Na+–K+–Cl− cotransporters functions as an anion importers, regulating trans-epithelial chloride secretion, cell volume, and renal salt reabsorption. Loop diuretics, including furosemide, bumetanide, and torsemide, antagonize both NKCC1 and NKCC2, and are first-line medicines for the treatment of edema and hypertension. Here we determined three cryo-EM structures of phosphorylated NKCC1 individually bound with furosemide, torsemide, and bumetanide, unlocking two modes of interaction of loop diuretics with NKCC1. In all the three co-structures, NKCC1 assembled as a C2-symmetric dimer in which two TMDs are separated by ~30 Å within the lipid bilayer and two cytosolic C-terminal domains (CTDs) interdigitate and associate extensively with the TMDs from beneath.

Furosemide intercalates into the NKCC1 extracellular ion entryway and assumes an extended configuration, with its sulfamoyl group facing the extracellular side and its furfuryl amine group reaching almost the midway of membrane. Notably, furosemide’s sulfamoylbenzoic moiety, which represents the molecular scaffold of carboxyl group-bearing loop diuretics, interacts extensively with residues in TM1, TM3, TM6, and TM8. Here, the chlorine atom barely contacts NKCC1, while the carboxyl group forms hydrogen bonds with Val302 and Met303 located on TM1b, and Ala497 residing on TM6a. The carboxyl group expels the Cl− ion from the so-called the Cl− site 1 and establishes ionic interaction with the K+ ion that was clearly seen to be co-occluded in the structure (Fig. EV3A). Further toward the midway of ion translocation path, furosemide’s furfuryl amine group is buried within a hydrophobic cavity and interacts with Met382 protruding from TM3, and IIe678, Ser679, and Phe682 which are all located on TM8. Indeed, we found that furosemide exhibits threefold higher potency in a K+ buffer than in a K+-free buffer. To settle this debate, we prepared pNKCC1 sample supplemented with 100 μM ATP and 2 mM furosemide, yielding an NKCC1/furosemide map in which we clearly observed a non-protein density that matches the shape of an ATP molecule in this cavity of NKCC1. In our pNKCC1/furosemide structure, ATP-Mg2+ binding stabilizes a loop (Gly925-Leu931) and a helix (Asn1002-Lys1021) that would otherwise be mobile and missing in all reported NKCC1 structures; the region which encompasses amino acids 932–1001 and contains sorting signals for trafficking NKCC1 to the basolateral membrane in epithelia remains unresolved. Our pNKCC1/furosemide map unambiguously defined the elusive N-terminal phosphoregulatory segment (residues Thr203-Leu250) which is seen to interact extensively with the swapped CTD of the second subunit and the intracellular loop 1 (ICL1; residues Thr343-Leu360) connecting the TM2 and TM3 helices.

>[2x]MEPRPTAPSSGAPGLAGVGETPSAAALAAARVELPGTAVPSVPEDAAPASRDGGGVRDEGPAAAGDGLGRPLGPTPSQSRFQVDLVSENAGRAAAAAAAAAAAAAAAGAGAGAKQTPADGEASGESEPAKGSEEAKGRFRVNFVDPAASSSAEDSLSDAAGVGVDGPNVSFQNGGDTVLSEGSSLHSGGGGGSGHHQHYYYDTHTNTYYLRTFGHNTMDAVPRIDHYRHTAAQLGEKLLRPSLAELHDELEKEPFEDGFANGEESTPTRDAVVTYTAESKGVVKFGWINGVLVRCMLNIWGVMLFIRLSWIVGQAGIGLSVLVIMMATVVTTITGLSTSAIATNGFVRGGGAYYLISRSLGPEFGGAIGLIFAFANAVAVAMYVVGFAETVVELLKEHSILMIDEINDIRIIGAITVVILLGISVAGMEWEAKAQIVLLVILLLAIGDFVIGTFIPLESKKPKGFFGYKSEIFNENFGPDFREEETFFSVFEIFFPAATGILAGANISGDLADPQSAIPKGTLLAILITTLVYVGIAVSVGSCVVRDATGNVNDTIVTELTNCTSAACKLNFDFSSCESSPCSYGLMNNFQVMSMVSGFTPLISAGIFSATLSSALASLVSAPKIFQALCKDNIYPAFQMFAKGYGKNNEPLRGYILTFLIALGFILIAELNVIAPIISNFFLASYALINFSVFHASLAKSPGWRPAFKYYNMWISLLGAILCCIVMFVINWWAALLTYVIVLGLYIYVTYKKPDVNWGSSTQALTYLNALQHSIRLSGVEDHVKNFRPQCLVMTGAPNSRPALLHLVHDFTKNVGLMICGHVHMGPRRQAMKEMSIDQAKYQRWLIKNKMKAFYAPVHADDLREGAQYLMQAAGLGRMKPNTLVLGFKKDWLQADMRDVDMYINLFHDAFDIQYGVVVIRLKEGLDISHLQGQEELLSSQEKSPGTKDVVVSVEYSKKSDLDTSKPLSEKPITHKVEEEDGKTATQPLLKKESKGPIVPLNVADQKLLEASTQFQKKQGKNTIDVWWLFDDGGLTLLIPYLLTTKKKWKDCKIRVFIGGKINRIDHDRRAMATLLSKFRIDFSDIMVLGDINTKPKKENIIAFEEIIEPYRLHEDDKEQDIADKMKEDEPWRITDNELELYKTKTYRQIRLNELLKEHSSTANIIVMSLPVARKGAVSSALYMAWLEALSKDLPPILLVRGNHQSVLTFYS> GPDPLPWCPHLESVRPVPAGGIDVFQPCEECGGEAENWICLFCYKVLCGRYVNQHMVTHGQESGHPVVLSFADLSVWCYA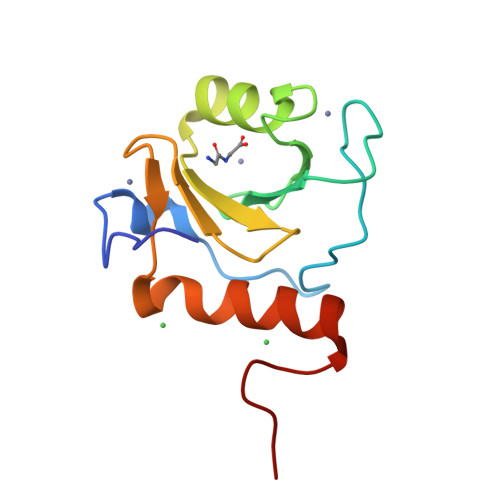CESYVHNKVLHEAKNAAHLVKFGEGIHPFN> XTVINLFAPGKVNLVEQLES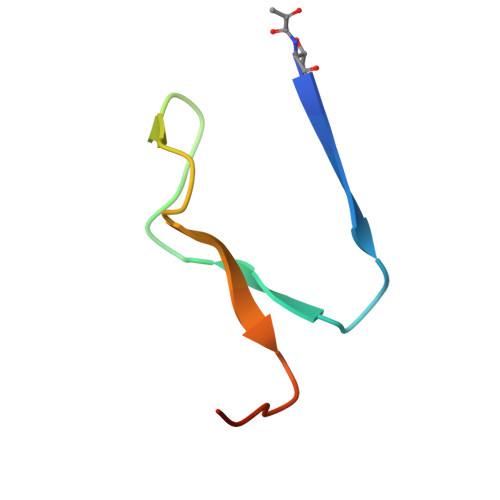LSVTKIGQPLAVSTGHHHHHHG> MANELTWHDVLAEEKQQPYFLNTLQTVASERQSGVTIYPPQKDVFNAFRFTELGDVKVVILGQDPYHGPGQAHGLAFSVRPGIAIPPSLL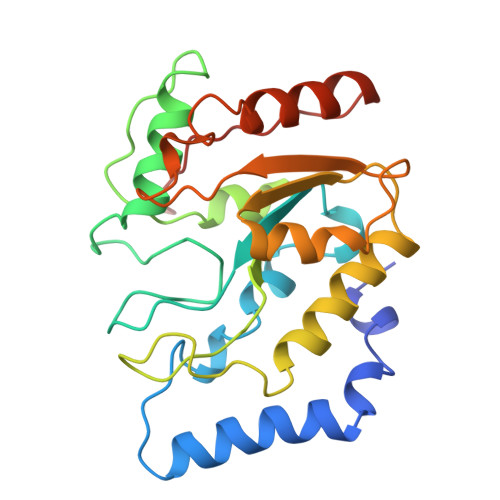NMYKELENTIPGFTRPNHGYLESWARQGVLLLNTVLTVRAGQAHSHASLGWETFTDKVISLINQHREGVVFLLWGSHAQKKGAIIDKQRHHVLKAPHPSPLSAHRGFFGCNHFVLANQWLEQRGETPIDWMPVLPAESE ChtII is a GH18 chitinase and possesses the greatest number of catalytic domains and chitin-binding domains in this family. Here we report the catalytic properties and the crystal structures of the catalytic domains of OfChtII, the ChtII derived from the Asian corn borer O. furnacalis. Analyzing the domain structure of the predicted protein with the SMART tool revealed that OfChtII contains five GH18 domains and seven CBM14-type chitin-binding modules (CBMs). The other two GH18 domains (C1 and C2) are predicted to be catalytically active (CAD).

OfChtII-C2 was also crystallized, and its crystal structure was resolved at a resolution of 1.95 Å. The P21 asymmetric unit comprised two molecules of OfChtII-C2 (which overlapped with an r.m.s. deviation of 0.24 Å over all atoms). OfChtII-C2 showed 60% sequence identity with OfChtII-C1. The overall architecture of OfChtII-C2 was very similar to that of OfChtII-C1, especially for the conserved (β/α)8 barrel domain (residues 2059–2301 and residues 2377–2426), corresponding to an r.m.s. deviation of 0.63 Å for 358 equivalent Cα atoms. However, subtle differences between OfChtII-C1 and OfChtII-C2 were observed. The entrance of the substrate-binding cleft in OfChtII-C2 was more open than that in OfChtII-C1.

>ERFKVVCYYTNWAWYRPDNGKYTPGDINPELCTHIIYAFAVLDKEELVIKSHDIWLDVENKFYEKVTALKSHGVKVLLGLGGWDDSAGDKYSRLVNNVSARRKFVVHAVDFLEQYGFDGLDLDWEYPKCWQVECEKGPDSDKQGFADLVKELRKAFNRRGMLLSAAVSASKRVIDYAYNVPALSMNLDWISLMTYDYHGQWDKKTGHVAPMYVHDKDTDNTFNVNFTVNYWINKGADRKKLVVGVPFYGQSFSVVEGAGTGLGAPTYAGGEAGDETRARGFLSFYEICERVKVKGWKVHRDPGGRIGPYATHDDQWVSFDDDFMARHKAEYVRAMELGGSMAWSLDLDDFTGKYCGCGKAPLLTTINHVLRGKEAPPPCILHE[2x]> IGGCRPSAQSLEIKHGDLSINSANNHYAAQTLSVSCDVPANIRFMLLRNTTPTYSHGKKFSVGLGHGWDSIVSVNGVDTGETTMRWYKAGTQNLTIGSRLYGESSKIQPGVLSGSATLLMIL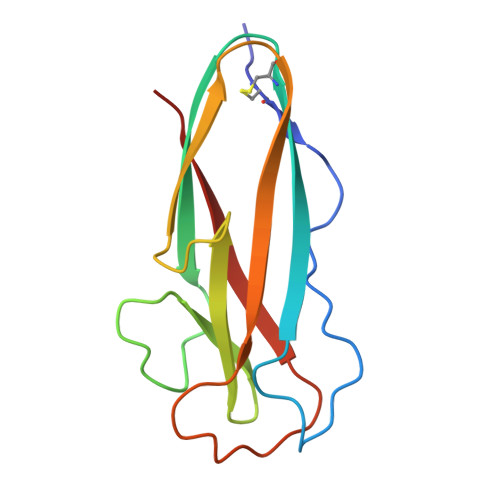P>MEFVAKLFKFFKDLLGKFLGNN[4x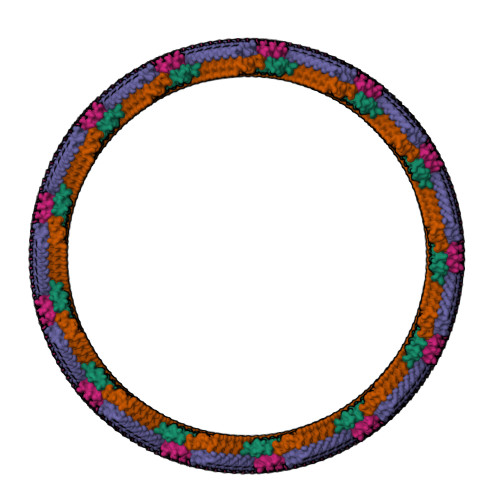]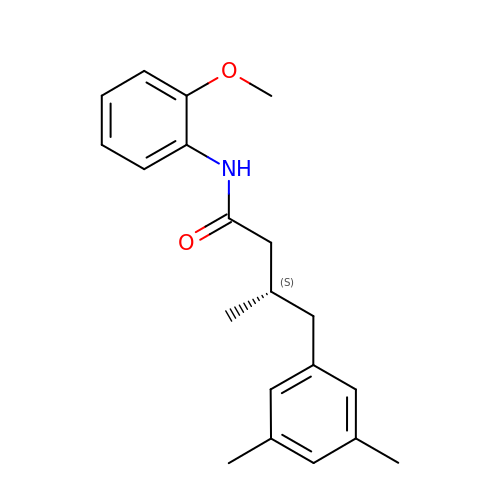(3S)-4-(3,5-dimethylphenyl)-N-(2-methoxyphenyl)-3-methylbutanamide | C20 H25 N O2 | XJYBAKSVSQKCNC-INIZCTEOSA-N> GAGCAGACCTGACG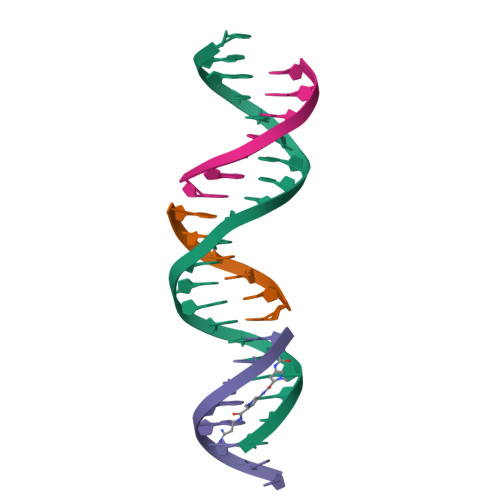GAAATTA;> CCGTCA;> TCTAATTT;> GGTCTGC>METILKMGLQANVGSVEYDSAKILSDKISELSDGEMKLLLYPGAQLGDDRAMLQQLSMGDLDITFAEFGRMGLWIPRAEAVMLPYVVKNYAHIQRIFNSKFGQGVREEMLTNFNWRALDTWYNGTRQTSSNRPLNTISDFEGLKLRVPNAKANLAFAKYAGASPTPMVFSEVYLALQTNAVDGQENPLPTFNTMKFYEVQPNLAMTNHIVNDQMVLISEDRWQSLSKDQQATITEAVSVAGKRHTNFVNNQEKELITFFKAEGVNITYPDLAPFREAMLPIYKDFDKKIGKQLVEELSDI[2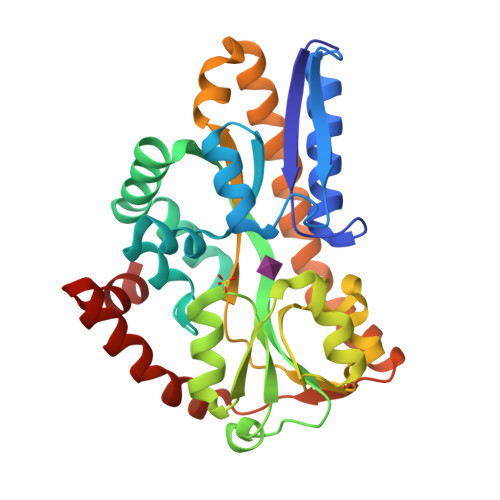x]>MPGSIPLIGERFPEMEVTTDHGVIKLPDHYVSQGKWFVLFSHPADFTPVSTTEFVSFARRYEDFQRLGVDLIGLSVDSVFSHIKWKEWIERHIGVRIPFPIIADPQGTVARRLGLLHAESATHTVRGVFIVDARGVIRTMLYYPMELGRLVDEILRIVKALKLGDSLKRAVPADWPNNEIIGEGLIVPPPTTEDQARARMESGQYRSLDWW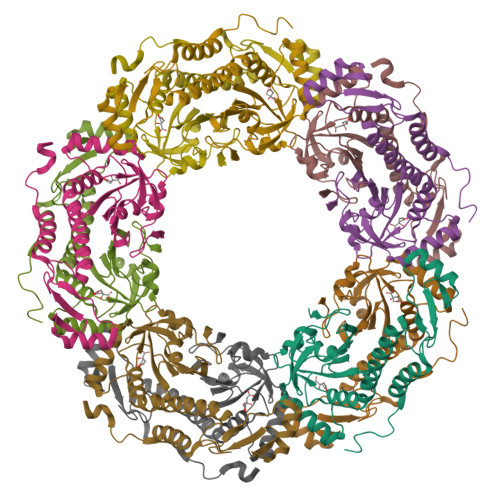FSWDTPASRDDVEEARRYLRRAAEKPAKLLYEEARTHLH[10x]> IVGGYTCGA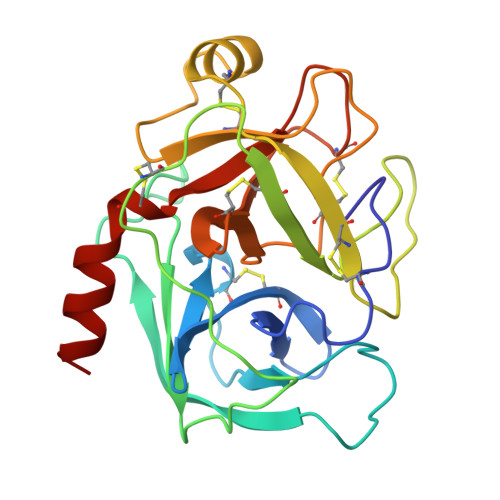NTVPYQVSLNSGYHFCGGSLINSQWVVSAAHCYKSGIQVRLGEDNINVVEGNEQFISASKSIVHPSYNSNTLNNDIMLIKLKSAASLNSRVASISLPTSCASAGTQCLISGWGNTKSSGTSYPDVLKCLKAPILSTSSCKSAYPGQITSNMFCAGYLEGGKDSCQGDSGGPVVCSGKLQGIVSWGSGCAQKNKPGVYTKVCNYVSWIKQTIASN>[4x]SNAMTDTVDFPDPSFGDRPNPVGWLDAHRMDEVRSLLPLVYVDAVPVRVDESGDVIQVGLLLRATESGHMMRALVSGRVMYHERVRDALVRHIEKDLGPVALPSIPASP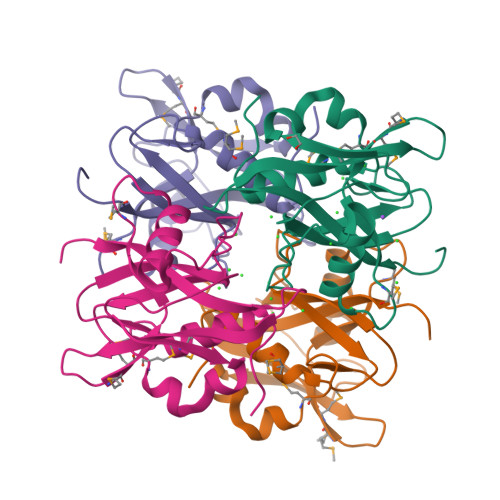QPFTVAEYFPTPGVTPFYDDRHHAVSLAYIVPVRGDCSPQQNNLELTWLTPEEACSPRILAHMQGGQDMLLKQALAHAGRLPDLS> XGPPGPKGDPGPKGDPGPPGARGQAGV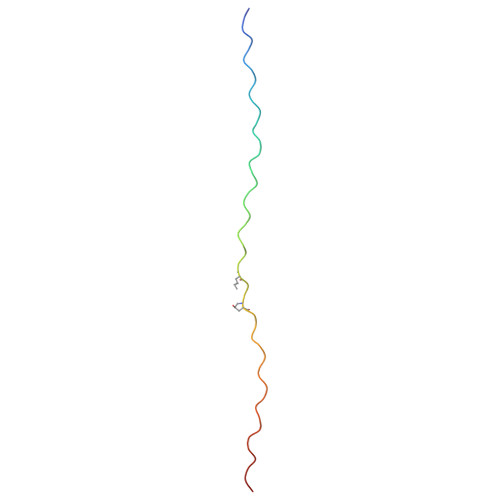LGFPGPPGPPGPKGDKGDPGGYX> MTMDEQQSQAVAPVYVGGFLARYDQSPDEAELLLPRDVVEHW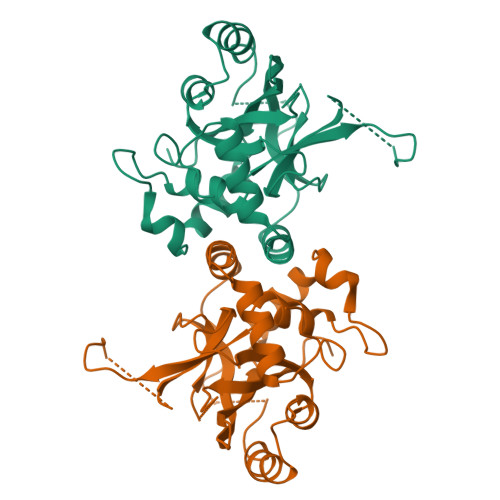LHAQGQGQPSLSVALPLNINHDDTAVVGHVAAMQSVRDGLFCLGCVTSPRFLEIVRRASEKSELVSRGPVSPLQPDKVVEFLSGSYAGLSLSSRRCDDVEVATSLSGSETTPFKHVALCSVGRRRGTLAVYGRDPEWVTQRFPDLTAADRDGLRAQWQRCGSTAVDASGDPFRSDSYGLLGNSVDALYIRERLPKLRYDKQLVGVTERESYVKA>[2x]SEEPPFDIRALRADIEDMISEKLELGPSLIRLAWHEAASYDCFKKDGSP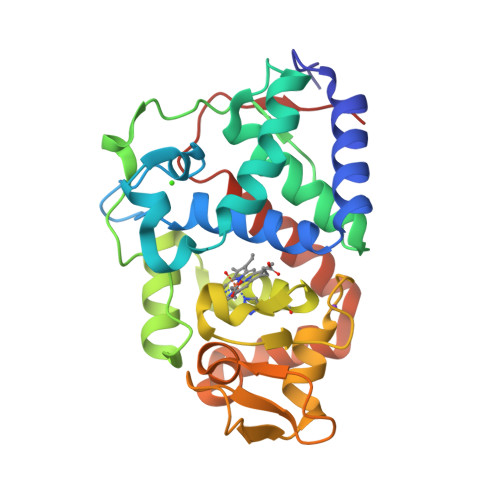NSASMRFKPECLYAGNKGLDIPRKALETLKKKYPQISYADLWVLAAYVAIEYMGGPTIPFCWGRVDAKDGSVCGPDGRLPDGSKTQSHVREVFRRLGFNDQETVALIGAHTCGECHIEFSGYHGPWTHNKNGFDNSFFTQLLDEDWVLNPKVEQMQLMDRATTKLMMLPSDVCLLLDPSYRKYVELYAKDNDRFNKDFANAFKKLTELGTRNLHKAPASES> ACGTCT;> GAACGACAAAGACGTCGAGTC;> TCGAGTCG;> TTGTCGT

In this work, we exhaustively probe the ability of all 36 immobile HJ sequences to form DNA crystals in two different designed systems. Three separate self-assembling DNA crystal systems are described in this report: the “4 × 5” and “4 × 6” designs (collectively referred to as the 4 × N systems), and a third construct with a “scrambled” sequence variant of the 4 × 6 lattices. Self-assembly was mediated by three constituent oligonucleotides: (S1) containing four sequence repeats of either 5 or 6 bases; (S2) composed of 21 bases containing complementary regions to both (S1); and (S3) which forms the second junction crossover. The HJ serves as the fundamental component at the core of each unit, and the ultimate assembly of the full lattice is facilitated by the complementary 2-base sticky ends that tail each duplex.

To investigate this possibility, we designed “scrambled” sequences with targeted base substitutions, while maintaining GC content, along each “stem”. Contrary to the buffer preference observed with the native P32 crystals, the scrambled systems exhibited an exclusive preference towards low salt buffers, much like the native R3 crystals. Remarkably, only J1 and J2 retained the P32 symmetry, with all others yielding an R3 lattice. There appeared to be only a marginal difference in the average cell lengths in the R3 scramble crystals (a = b = 113.04 c = 51.10) relative to the native 4 × 6 sequences: the a, b axis trended ~2 Å shorter and c ~1.3 Å longer, whereas in the J1 and J2 cases, the crystals were in good agreement with the original 4 × 6 motif. The average angles of the R3 and P32 crystals were 61.00° (σ = 1.21) and 58.05° (σ = 1.39), respectively. Another major observation is the importance of stem region sequences outside the HJ, given that this sequence can control crystal symmetry and lattice architecture, and improve resolution in non-obvious ways. However, in the majority of the crystal structures reported here, the cacodylate anion indeed fits best into the electron density map of our X-ray structures, due to the presence of sodium cacodylate in the crystallization solution.>SASIEKVNKLPKSPRNRFLLPPKGGTETTRRDIYNQILKDMAAFPENTIVTAVLASVDVTDNCAYVAKWDESSDRIKKVLQRQLPLQELDQLPDYGDIFAVLDSINNIITRITINSSSAGGGYDAYLIDFGEHIHFDGNETIFKLPDDIKRLPAQAIRCDLINCDIANMHCFVNTYIKIRVHENNNSTLVAEPVIDRLSRPTKTNTTKYPAGITEDDMAMLNEID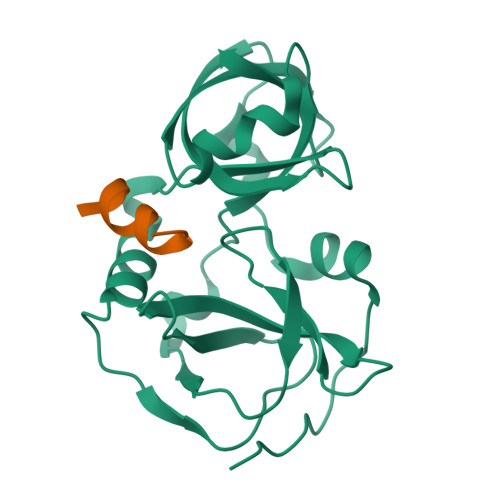ESTSDPLKAVLGFRPKD[5x];>[4x]NISVGRGRARLIDTLK> GAASKKVNVLVVGLDNSGKTTIIERLKPRPRQAA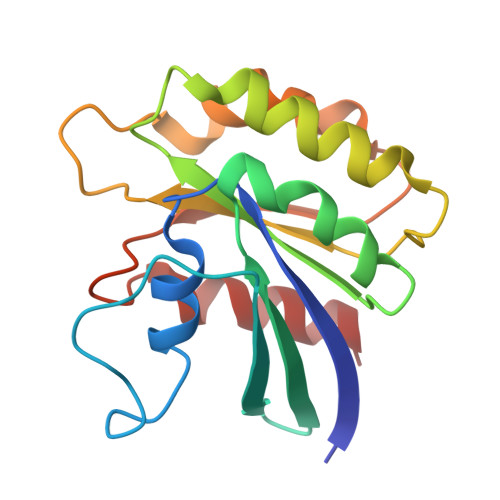EVAPTVGFTVDEVEKGPLTFTVFDMSGAGRYRTLWEQYYREADAVVFVVDSADKLRMVVARDEMEHMLKHSNMRKVPILYFANKKDLPVAMPPVEIAQALGLDDIKDRPWQIVPSNGLTGEGVDKGIDWLAERLS>[8x]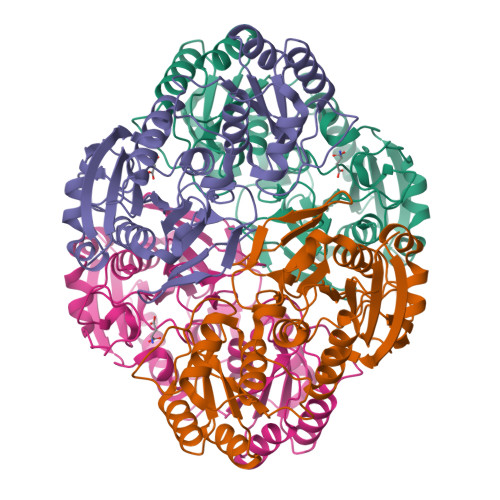AENLPNIVILATGGTIAGSAAANTQTTGYKAGALGVETLIQAVPELKTLANIKGEQVASIGSENMTSDVLLTLSKRVNELLARSDVDGVVITHGTDTLDESPYFLNLTVKSDKPVVFVAAMRPATAISADGPMNLYGAVKVAADKNSRGRGVLVVLNDRIGSARFISKTNASTLDTFKAPEEGYLGVIIGDKIYYQTRLDKVHTTRSVFDVTNVDKLPAVDIIYGYQDDPEYMYDASIKHGVKGIVYAGMGAGSVSKRGDAGIRKAESKGIVVVRSSRTGSGIVPPDAGQPGLVADSLSPAKSRILLMLALTKTTNPAVIQDYFHAY> MSEYMDDVDREFINCLFPSYLLQQPVAYDLWILYLQHRKLFHKLKNTNLINADENPTGVGMGRTKLTALTRKEIWSKLMNLGVLGTISFEAVNDDYLIQVYKYFYPDVNDFTLRFGVKDSNKNSVRVMKASSDMRKNAQELLEPVLSEREMALNSNTSLENDRNDDDDDDDDDDDDDDDDDDDDDESDLESLEGEVDTDTDDNNEGDGSDNHEEGGEEGSRGADADVSSAQQRAERVADPWIYQRSRSAINIETESRNLWDTSDKNSGLQYYPPDQSPSSSFSSPRVSSGNDKNDNEATNVLSNSGSKKKNSMIPDIYKILGYFLPSRWQAQPNNSLQLSQDGITHLQPNPDYHSYMTYERSSASSASTRNRLRTSFENSGKVDFAVTWANKSLPDNKLTIFYYEIKVLSVTSTESAENSNIVIGYKLVENELMEATTKKSVSRSSVAGSSSSLGGSNNMSSNRVPSTSFTMEGTQRRDYIYEGGVSAMSLNVDGSINKCQKYGFDLNVFGYCGFDGLITNSTEQSKEYAKPFGRDDVIGCGINFIDGSIFFTKNGIHLGNAFTDLNDLEFVPYVALRPGNSIKTNFGLNEDFVFDIIGYQDKWKSLAYEHICRGRQMDVSIEEFDSDESEEDETENGPEENKSTNVNEDLMDIDQEDGAAGNKDTKKLNDEKDNNLKFLLGEDNRFIDGKLVRPDVNNINNLSVDDGSLPNTLNVMINDYLIHEGLVDVAKGFLKDLQKDAVNVNGQHSESKDVIRHNERQIMKEERMVKIRQELRYLINKGQISKCINYIDNEIPDLLKNNLELVFELKLANYLVMIKKSSSKDDDEIENLILKGQELSNEFIYDTKIPQSLRDRFSGQLSNVSALLAYSNPLVEAPKEISGYLSDEYLQERLFQVSNNTILTFLHKDSECALENVISNTRAMLSTLLEYNAFGSTNSSDPRYYKAINFDEDVLNL;> MINNPKVDSVAEKPKAVTSKQSEQAASPEPTPAPPVSRNQYPITFNLTSTAPFHLHDRHRYLQEQDLYKCASRDSLSSLQQLAHTPNGSTRKKYIVEDQSPYSSENPVIVTSSYNHTVCTNYLRPRMQFTGYQISGYKRY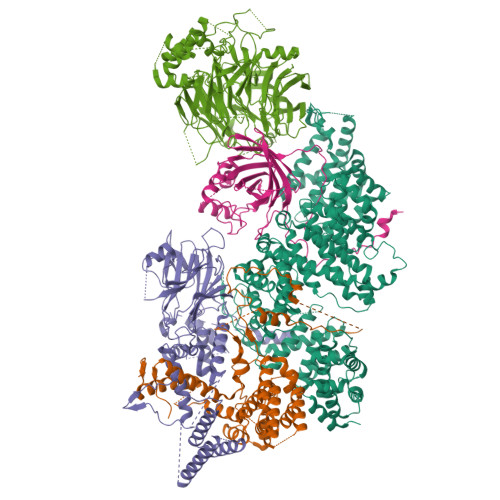QVTVNLKTVDLPKKDCTSLSPHLSGFLSIRGLTNQHPEISTYFEAYAVNHKELGFLSSSWKDEPVLNEFKATDQTDLEHWINFPSFRQLFLMSQKNGLNSTDDNGTTNAAKKLPPQQLPTTPSADAGNISRIFSQEKQFDNYLNERFIFMKWKEKFLVPDALLMEGVDGASYDGFYYIVHDQVTGNIQGFYYHQDAEKFQQLELVPSLKNKVESSDCSFEFA;> MTVAYSLENLKKISNSLVGDQLAKVDYFLAPKCQIFQCLLSIEQSDGVELKNAKLDLLYTLLHLEPQQRDIVGTYYFDIVSAIYKSMSLASSFTKNNSSTNYKYIKLLNLCAGVYPNCGFPDLQYLQNGFIQLVNHKFLRSKCKIDEVVTIIELLKLFLLVDEKNCSDFNKSKFMEEEREVTETSHYQDFKMAESLEHIIVKISSKYLDQISLKYIVRLKVSRPASPSSVKNDPFDNKGVDCTRAIPKKINISNMYDSSLLSLALLLYLRYHYMIPGDRKLRNDATFKMFVLGLLKSNDVNIRCVALKFLLQPYFTEDKKWEDTRTLEKILPYLVKSFNYDPLPWWFDPFDMLDSLIVLYNEITPMNNPVLTTLAHTNVIFCILSRFAQCLSLPQHNEATLKTTTKFIKICASFAASDEKYRLLLLNDTLLLNHLEYGLESHITLIQDFISLKDEIKETTTESHSMCLPPIYDHDFVAAWLLLLKSFSRSVSALRTTLKRNKIAQLLLQILSKTYTLTKECYFAGQDFMKPEIMIMGITLGSICNFVVEFSNLQSFMLRNGIIDIIEKMLTDPLFNSKKAWDDNEDERRIALQGIPVHEVKANSLWVLRHLMYNCQNEEKFQLLAKIPMNLILDFINDPCWAVQAQCFQLLRNLTCNSRKIVNILLEKFKDVEYKIDPQTGNKISIGSTYLFEFLAKKMRLLNPLDTQQKKAMEGILYIIVNLAAVNENKKQLVIEQDEILNIMSEILVETTTDSSSYGNDSNLKLACLWVLNNLLWNSSVSHYTQYAIENGLEPGHSPSDSENPQSTVTIGYNESVAGGYSRGKYYDEPDGDDSSSNANDDEDDDNDEGDDEGDEFVRTPAAKGSTSNVQVTRATVERCRKLVEVGLYDLVRKNITDESLSVREKARTLLYHMDLLLKVK;> MTISTLSNETTKSGSCSGQGKNGGKDFTYGKKCFTKEEWKEQVAKYSAMGELYANKTIHYPLKIQPNSSGGSQDEGFATIQTTPIEPTLPRLLLNYFVSMAYEDSSIRMAKELGFIRNNKDIAVFNDLYKIKERFHIKHLIKLGRINEAMEEINSIFGLEVLEETFNATGSYTGRTDRQQQQQQQQFDIDGDLHFKLLLLNLIEMIRSHHQQENITKDSNDFILNLIQYSQNKLAIKASSSVKKMQELELAMTLLLFPLSDSADSGSIKLPKSLQNLYSISLRSKIADLVNEKLLKFIHPRIQFEISNNNSKFPDLLNSDKKIITQNFTVYNNNLVNGSNGTKITHISSDQPINEKMSSNEVTAAANSVWLNQRDGNVGTGSAATTFHNLENKNYWNQTSELLSSSNGKEKGLEFNNYYSSEFPYEPRLTQIMKLWCWCENQLHHNQIGVPRVEN;> MATGRIQFAVSTPCNTKGKPSGYRLFEFKNDRLALVPSERGCTKVDVNANIQAFCYLRPNGRDTSISPDATHILDSCDYMVLAKSNGFIEIISNYQYKIKNGLRLAPSYILRCTPEDFESNFFSDYMIAGLEYSQGLLYCCMCSGRIYVFVMNLPTDYIQYKNMYNPMFPDCFFKVHHDNNTTHSSEEEKLFEGSTRYTGRSCSKHICYFLLPIEPSHLRSSPVVSSFCNMYQGLPIYRPSMYLHIERGISTFHINPLDRFCFMTVSPRSPLFIRKIILPLTYVTFLSTFISLKNSIQGDTCGEILSWDNVAQQNGFGSLFSWISNKFTFDTDIINSTIWDDIVKYSGTGMLDSGIVWKQRQGHAKDDIYELFHTQDMLGSSRRNSSFSTASSEPRPLSRRRRESFQALTRDAFRERMDVPCSTKWELDSFIRGLRRNTFMVDFEIVEKISHRNGNDGVNEDDNTTDESDETMTSFLTDNYKKMDIVCIDHFVTLSAFRPRYYDEPIIKIDSLSNKNGSENGTNEEEWAESQMKVDGQVIDDETAQFKQALGNLCSFKKLFMLDDSLCFILDTHGVLLINRFEIKNTKNLLRNSKDTIRIIPHDFGLINDTIVIINDIDVGTDNVCALTFHLVVTSMAGEITVLKGEFFKNCRLGRIKLCDSLKLNRKDRFVDKLALIDYDGLNAQKRRLDYDEKDLYTFIVKKVKRD> GGSE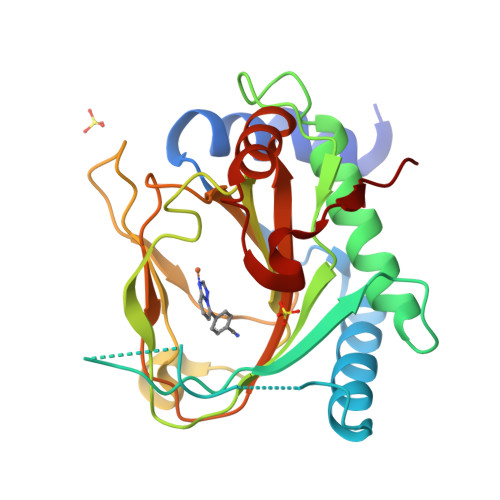EALPSAPERLALDYIVPCMRYYGICVVDSFLGAALGGRVLAEVEALKRGGRLRDGQLVSQRAIPPRSIRGDQIAWVEGHEPGCRSIGALMAHVDAVIRHCAGRLGSYKINGRTKAMVACYPGNGLGYVRHVDNPHGDGRCITCIYYLNQNWDVKVHGGLLQIFPEGRPVVANIEPLFDRLLIFWSDRRNPHEVKPAYATRYAITVWYFDADERARAKDKYQLASGQKGVQVPVSQP> VSEKQLAEVVANTVTPLMKAQSVPGMAVAVIYQGKPHYYTFGKADIAANKPVTPQTLFELGSISKTFTGVLGGDAIARGEIS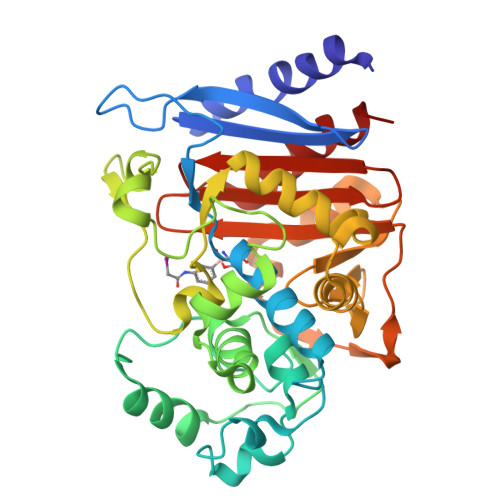LDDPVTRYWPQLTGKQWQGIRMLDLATYTAGGLPLQVPDEVTDNASLVRFYQNWQPQWKPGTTRLYANASIGLFGALAVKPSGMPYEQAMTTRVLKPLKLDHTWINVPKAEEAHYAWGYRDGKAVRVSPGMLDAQAYGVKTNVQDMANWVMANMAPENVADASLKQGIALAQSRYWRIGSMYQGLGWEMLNWPVEANTVVEGSDSKVALAPLPVVEVNPPAPPVKASWVHKTGSTGGFGSYVAFIPEKQIGIVMLANTSYPNPARVEAAYHILEALQ N-{2-chloro-5-[(3S,4R)-1-[(3R)-4-(4-chlorophenyl)-3-hydroxybutanoyl]-4-(hydroxymethyl)pyrrolidin-3-yl]phenyl}-2-(4-fluorophenyl)acetamide 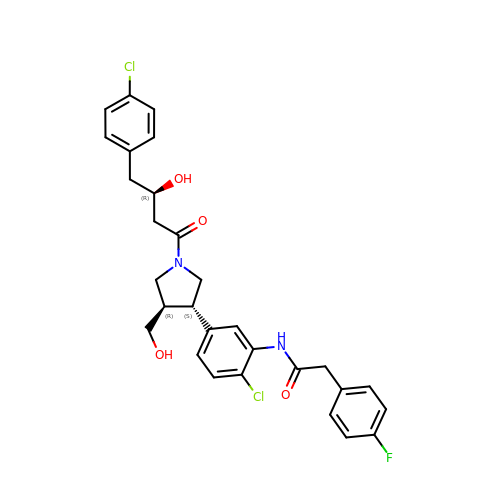| C29 H29 Cl2 F N2 O4 | LMARVLAZWJAMGJ-NQHRYMMQSA-N>[2x]MKDLVDTTEMYLRTIYELEEEGVTPLRARIAERLEQSGPTVSQTVARMERDGLVVVASDRSLQMTPTGRTLATAVMRKHRLAERLLTDIIGLDINKVHDEASRWEHVMSDEVE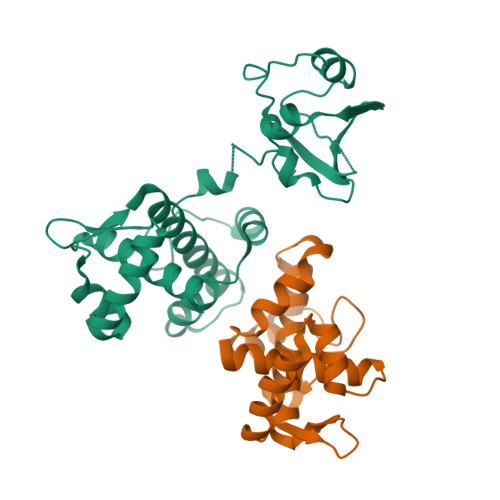RRLVKVLKDVSRSPFGNPIPGLDELGVGNSDAAAPGTRVIDAATSMPRKVRIVQINEIFQVETDQFTQLLDADIRVGSEVEIVDRDGHITLSHNGKDVELLDDLAHTIRIEEL>MNFRTLPDGVSAEQFANAISEFSETIGSEYVRVDEATVSEYDDKFPVTDGDEFKGSAVIWPGSTEDVQVIVRIANKYGIPLHAFSGGRNLGYGGSSPMLTGTVLLHLGKRMNRVLEINEKLAYAVVEPGVDYKTLYEAVRDSGAKLMIDPAELDWGSVMGNTMEHGVGYTPYADHSMWRCGMEVVLADGEVLRTGMGGLPGSEAWHLYPGQLGPSIEGLFEQSNFGICTRMGMQLMPTPPEMLSFAIYFENEDDLPAIMETTLPLRIGMAPLQAAPIVRNVTFDAACVSKREEWQTEPGPLTDEAKQRMVDELGIGHWIVYGTCYGPRWQIDKYIEMIRDAYLQIPGARFETNETLPLREGDRASELLNARHELNTGVPNRHSAAVFDWFPNAGHFFYAPVSAPSGEDAAKQYEDTKRISDDHGIDYLAQFIIGLREMHHICLPLYDTADPASRKETLDMTRELIRAGAEEGYGIYRAHNVLADQVAETYSFNNHIQRRSHERIKDALDPNGILNPGKS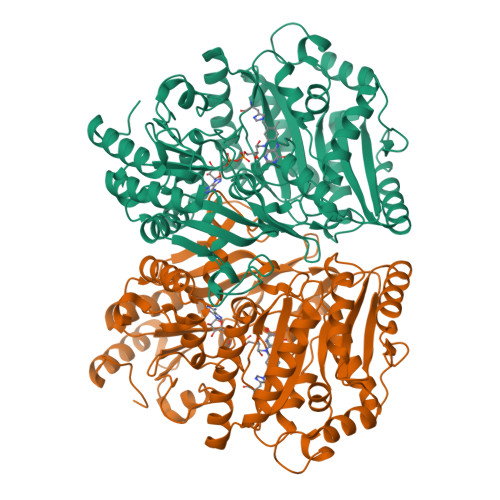GIWPERLRNK[8x]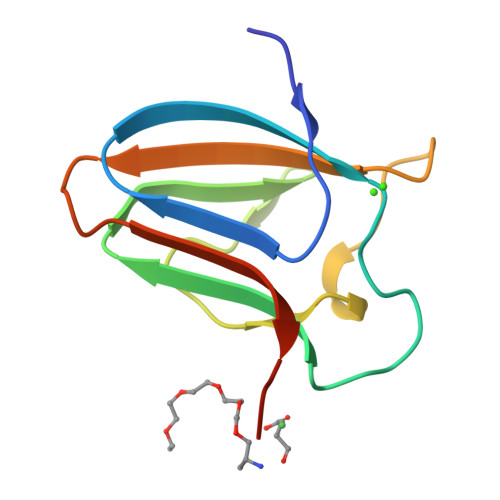> GEYLEMDLPFSYDGAGEYLWKTDDFSTTVDWGRYVNSWNLDLLEINGNDYTNRWVAQHQVPPASDGYWYIHYKGSLAWSHVEMKLEHHHHHH MetX (previously mis-annotated as MetA in the reference genome of M. tuberculosis) is an l-homoserine O-acetyltransferase, commonly also referred to as a homoserine transacetylase (HTA) and is a crucial enzyme in the biosynthesis of methionine and threonine. Here we report the structures of three homologous MetX enzymes from Mycobacterium tuberculosis (MtMetX), Mycolicibacterium abscessus (MaMetX), and Mycolicibacterium hassiacum (MhMetX) and compare them to previously solved structures of HTAs in order to begin development of selective inhibitors of MtMetX via a structure-based approach. Two copies of each monomer exist in the asymmetric unit of all three structures. MetX can be divided into two distinct structural domains, the catalytic domain, and the lid domain. The organization of the catalytic domains’ fold marks MetX as members of the α/β-hydrolase super-family.

The three solved MetX structures include residues 15–70, 77–372 from MhMetX, 10–379 from MaMetX, and 7–372 from MtMetX. The catalytic domain comprises residues 15–181, 297–372 of MhMetX, residues 17–183, 304–379 of MaMetX and residues 17–181, 311–372 of MtMetX. For MtHTA and MhHTA, Ser157, Asp320, and His350 comprise the active site; MaHTA’s triad is comprised of Ser160, Asp327, His357. MtMetX and MsHTA both contain a small helical region (αL1′); MaHTA features a unique pair of short anti-parallel sheets (β1′, β2′). Interestingly, MsHTA is as good if not better an approximation to MtMetX as either MhMetX or MaMetX, suggesting that it may function as a good analog in assays where MtMetX cannot be directly utilized. However, when assaying MtMetX to determine its viability for crystallography, the Tm was found to be between 40–41 °C by differential scanning fluorimetry (DSF) between pH 6.9–8.5 in Tris-HCl. Because of MtMetX’s relative thermal stability under physiological conditions, we have chosen to focus on MtMetX when investigating future drug development. Using the MtMetX structure as a guide, we also elucidate the druggability of the enzyme and propose that it is an excellent candidate for small molecule drug discovery. Of the eleven CS identified by FTMap, eight reside somewhere within the active site tunnel. The closest CS near the catalytic Ser have S = 19, S = 16 and S = 13.

>[2x]GAMTLPAEGEIGLIDVGSLQLESGAVIDDVCIAVQRWGKLSPARDNVVVVLHALTGDSHITGPAGPGHPTPGWWDGVAGPGAPIDTTRWCAVATNVLGGCRGSTGPSSLARDGKPWGSRFPLISIRDQVQADVAALAALGITEVAAVVGGSMGGARALEWVVGYPDRVRAGLLLAVGARATADQIGTQTTQIAAIKADPDWQSGDYHETGRAPDAGLRLARRFAHLTYRGEIELDTRFANHNQGNEDPTAGGRYAVQSYLEHQGDKLLSRFDAGSYVILTEALNSHDVGRGRGGVSAALRACPVPVVVGGITSDRLYPLRLQQELADLLPGCAGLRVVESVYGHDGFLVETEAVGELIRQTLGLAD>[4x]GP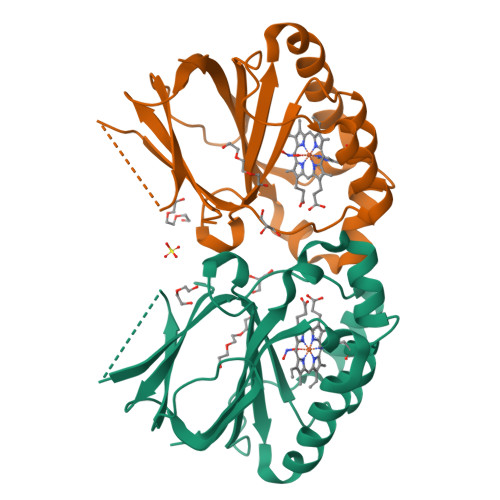GYQDPNNRYSFIGGRTGQWQVVKIRNVLGPGLQLVEKVNILNGAVAEIPLDSAWRLQGFASNIRYAIRTELEALQAVQPMLNRAEAILAVLIPIKKSAQWWEMAQDERRDIFERESHHTAVGLEYLPGVAARLLHCRDLGEEFDFLTWFEFAPEHSSAFNELLLRMRASKEWEYVEREVEVWLKRL> NASGERLSQLLKKLFETQESGDLNEELVKAAANGDVAKVEDLLKRPDVDVNGQCAGHTAMQAASQNGHVDILKLLLKQNVDVEAEDKDGDRAVHHAAFGDEGAVIEVLHRGSADLNARNKRRQTPLHIAVNKGHLQVVKTLLDFGCHPSLQDSEGDTPLHDAISKKRDDILAVLLEAGADVTITNNNGFNALHHAALRGNPSAM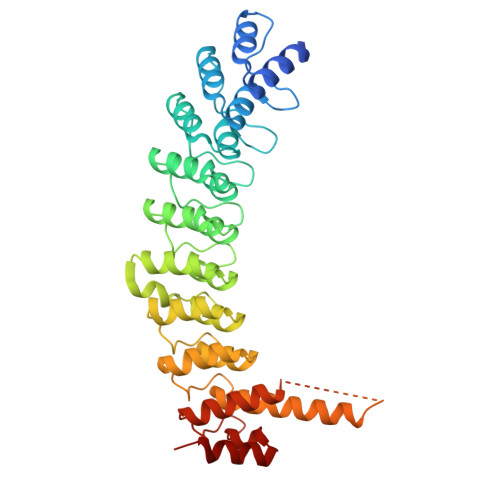RVLLSKLPRPWIVDEKKDDGYTALHLAALNNHVEVAELLVHQGNANLDIQNVNQQTALHLAVERQHTQIVRLLVRAGAKLDIQDKDGDTPLHEALRHHTLSQLRQLQDMQDVGKVDAAWEPSKNTLIMGLGTQGAEKKSAASIACFLAANGADLSIRNKKGQSPLDLCPDPNLCKALAKCHK>MVESDSSGIVRHSQGEFDIVQVYKKFLQDDPEITMPVAAIEALVQLLSRSQAKTISEFMDILQNGSNTLKEGVQNNISLSAGCDIFQRFVTRSLHDVGDFEQCKRHLVENGKLFIQRARACRQRIAHLGYPLIRDGSVILTHGFSRGVAAVLLAAAKRHVRFKVFVTESRPSGSGCLMTRTLKNACIPTCMVLDSAVSFTMNRVDLVLVGAEGVVENGGLINQIGTFQLAVFAKHAHKPFYAVAESHKFVRMFPLSQYDIPFSRPILEFDDPSPETVHPEPEPIPTPSDAIHNELIMNEEQIRNNPTLDVTPPEFVSGLITDLGIIDSKSGVSEELIKLYL[2x];>GPISEFMSTINVEHTYPAVSSLIADLKSRKVQGPFAVAVETALVMRQVISQTRWSTVDQLIDTVRAVGSTLVKAQPTEFSCGNIIRRILRLIREEYQELLKTADENEKLIVSSSNSSSPSQKRDIPSNEKLVQSHEPVSVQMYSSMLNLLGRPTLESPTHSKTVGDSRVTGGMDMRAVIISGIQDVIDELDKINTDIEVQSMDHLHSNEIILTQGCSKTVEAFLRFAAKKRKFSVIVAEGFPNNQKGSHAMAKRLAQAGIDTTVISDATIFAIMSRVNKVILGTHAILGNGGLVTYSGAQLVAQAARHHATPVVVCSGIYKLSPVYPYDLESIIQLSSPDKIMSFNEGDLISRAEILNPYYDYIPPDLVDLFITNLGGYPPSYLYRIMNDTYDASDTIL[2x];>[2x]MSLYEHAALPLASSPSILGPISGGRNRGNIQLQSIPIEFQAVVFAGFGNSLYPLTGSDALPKALLPIGNKPMLHYPLYWLEAAGFTSAILICMEEAEAHINAWLRSGYEGHMRIHVEAPTILDDSKSSADALRAVSHLIKNDFVCLSCDSIVGLPPYTVLDKFRLDNPSALAVYSPVLKYEHITSQSKEIDAKQLIGIEEKTSRLLYAKSSADVGSDFTFRMSLLWKHPRVTLNTNLSDAHIFVFKHWVIDLIREKESISSIRGDLIPYLVKCQYQKSFTVRENIQRFLSSPNNIDNYDGGLSS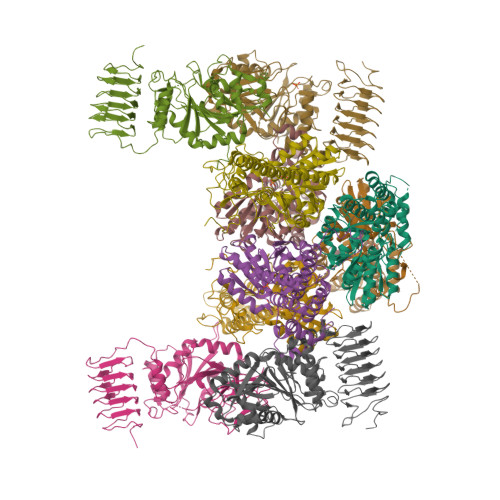QEIKINALIAKDGIICSRANNLPNYFELNKCIAKLTPEQRLVDVTVSERALVGADCMVNEGTTIKDNSNIKKSIIGKNCVIGKGVVVSNSILMDNIVVEDGVRLESCIVASGAQIGAKSKLRECEIGVDHRVEAGRIARGERLVDMEKIETDMD;>[2x]MGFSAEQAKKDGKDQSPVSESSSVGGTSPATASSVVSPNEPKLSGKEAKALKKARKQASRRAKAEAAAANNPPGVSEEKKVAIPNKNSNQQKKASKQNPQNSPETDANLQEKKIFEEKQVSIFSHLDWRRRRTTENIPKDIHPAVIRLGLKLANYKIFGSNQRCIDLLKTFKIVIQDYQTPYGTTLSRHLTTHINSQIAYLVSTRPLSISMGNAIRFLKLEISVLDIDLTDDEGKELLLEKIDSYIRDRIIIAGQVIVQAATEKIQDGDVILTYLHSSTVNDVLIHAKNVGKKFRVVVVDSRPEFEGRVCLKLLTEHGIECTYVMISALSYIMQEVTKIFLGGHAMLSNGALYSRAGTSLISLLGHESNVPVIACCESYKFTERIQLDSLVYNELAPGDQLVNMGVDDFEEKPGVLANWKSVKNLKLLSLKYDVTPPRLITVCVCEMGLLPSTSVPAIINEFKQVYA;>[2x]MPPSKGLNGKLEKPKHALQAIVLSDSYNYRFRPLTLDKPRCLLPLANTPLIEYTFEFLALAGVQEVYVFCCAHAGQIREYIEKSKWNLPSSPFSVNTIVSRESLSVGDALRELDSKQLITSDFILVSGDVVSNVPLNEVLKEHRKRREDDKNAIMTMVVREASPFHRTRARTESSVFVIDKKTSQCVHYQANERGKHYVSMDPEIFNEHEELEVRNDLIDCQIDICSNDVPALFTENFDYQDIRKDFVYGVLTSDLLGKKIHCHVAKENYAARVRSLQTYDAISKDVLSRWVYPFVPDSNLLNQTFSYQRHQIYKEEDVVLARSCIIKARTLIGAYTKVGDASVVANTIIGRNCTIGSNCSIDSAFLWEDVVIGDNCRIGKAILANSVKIGNNCSIEDGAIVAAGVVIGDNTIIEKNKRLTTFESHSQGTLNDPSLVGIGGRGQEYHAEEDSDDEGEFMEASGLIESTNELHLSDSESSETSSSSEEDMEFIPFSARRDSANTINSEDFDEGDFNKEAQQSLERAFEENHQIDIAALELNTLRMAMNANYHEVRSAIVLALLRRIMHLDVSPKEALAKVMTRWGPLLAKLTFSHEEQVDNVLTLQKYCVRLSMTRHFLQLLGYFYQLEIAEENAIQEWYSDPRSSEGELAALRDAGGKQFVDWLNTAESESESEEGSE>[2x]MGHHHHHHMVLMTKPGTSDFVWNGIPLSMELNLWNIKEYSGSVAMKFDGEKITFDADIQNLSPKEPERGGVLGYPEFYYGYKPWENHTAEGSKLPVPVSSMKSFSVEVSFDIHHEPSLPLNFAMETWLTREKYQTEASIGDVEIMVWFYFNNLTPGGEKIEEFTIPFVLNGESVEGTWELWLAEWGWDYLAFRLKDPVKKGRVKFDVRHFLDAAGKALSSSARVKDFEDLYFTVWEIGTEFGSPE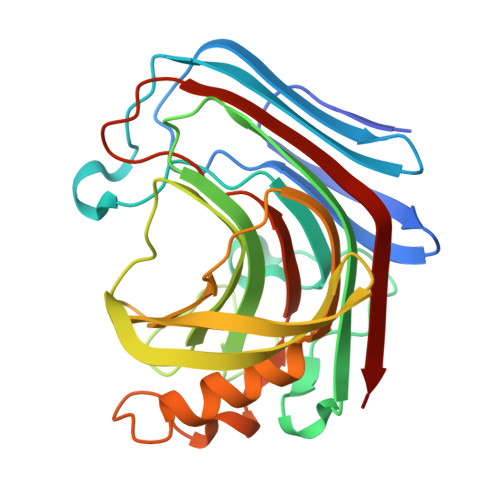TKSAQFGWKFENFSIDLEVRE> SHMNKDNLRSPICCILGHVDTGKTKLLDKIRQTNVQEGEAGGITQQIGATYFPVEAIKQKTAVVNKDGKFEFKVPGLLIIDTPGHESFSNLRSRGSSLCNIAILVVDIMHGLEPQTIESLRLLRERKTPFVVALNKIDRLYGWKKIENNGFRESFALQNKAVQNEFRNRLDQVKLQFAEQGFNSELFYENKNFARYVSLVPTSAHTGEGIPDMLKLIVQLCQERMASSLMYLSELQATVLEVKAIEGFGVTIDVILSNGILREGDRIVLCGLEGPIKTNIRALLTPAPMRELRIKGQYIHHKEVKAAQGVKISAPGLEGAIAGSRLLVVGPDDDEEELEEEVESDLQSLFSRVEKTGKGVSVQASTLGSLEALLDFLKDCKIPVANVGIGPVYKRDVMQCGIMLEKAPDYAVMLCFDVKVDKEAQQYADENGIKIFTADIIYHLFDQFTKHMQEQLEKKKEESKMLAVFPCVLNPVAVFNKTNPIVVGVDVVDGQLKLNTPIAAVKMNPTTGQKEIISLGRVTGIERDHKPLQVCKKGQPAVAIKIEMGGHQPAYGRHLDEKDVLYSHISRASIDVLKQFYRDVVTTDEWQLIIKLKSVFDV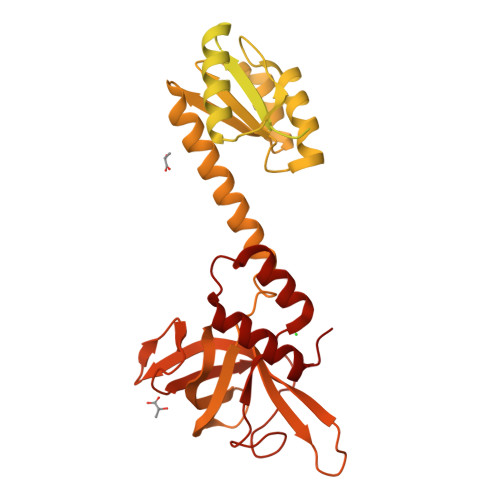Q HEXANE-1,6-DIAMINE | C6 H16 N2 | 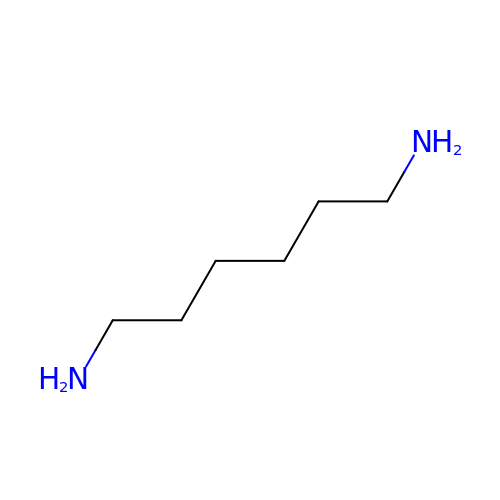NAQMVNRVTILPCV-UHFFFAOYSA-N>[2x]MLAPADKNKRQDELIVLNVSGRRFQTWRTTLERYPDTLLGSTEKE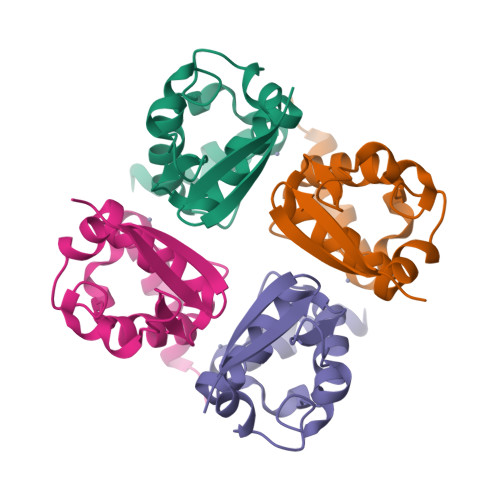FFFNEDTKEYFFDRDPEVFRCVLNFYRTGKLHYPRYECISAYDDELAFYGILPEIIGDCCYEEYKDRKRENLEHHHHHH> MTERRHDREFVRTFFTSPTAVEGEDDSAKMLRRAAGLRGMQAPDVWVPDNEDATAPSMRDEGAENIVEVISEQGAEFPGEIHPRMVWHRDSPETRYQGFQHMLDITDPERGAVEHIHGFVIPEVGGIDDWKKADEFFTIVEHEHGLDEGSLAMSVIIES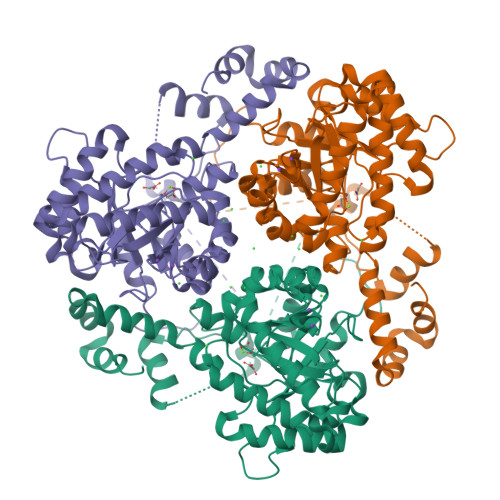GEAELAMGDLRDEMGKPTNNLERLFLLVDGEVDYTKDMRAMTPTGELPAWPELRHNTSRGASAAGCVAVDGPYDDIRDVEGYRERMTDNQAKGMLGIWSLTPGQVVEANTSPLPPKTGSWLLDADGEEVELASEDGVEAYDGDRLSLEATDGGYELRVGGDARELTADELREELLGLTSYVPSMDDIVDSMEEFEAAKEAGRGAIAMTQSATLRIGGTEIDIEKDRMWDEATYQAAMTPISLFQDVYENRPDQHEELEERYGAGVVERAMEVGL>[4x]GSMSTLL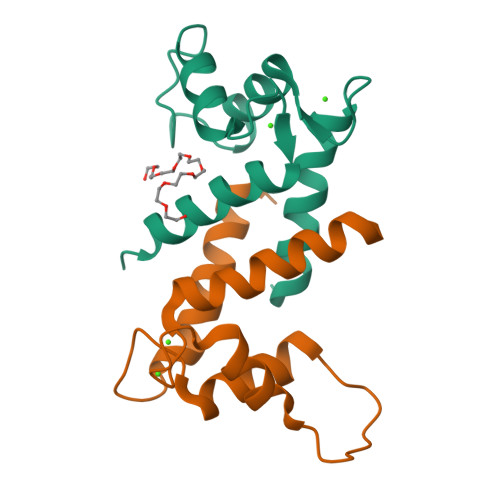ENIFAIINLFKQYSKKDKNTDTLSKKELKELLEKEFRQILKNPDDPDMVDVFMDHLDIDHNKKIDFTEFLLMVFKLAQAYYESTRKE S-[2-[3-[[(2R)-4-[[[(2R,3S,4R,5R)-5-(6-aminopurin-9-yl)-4-oxidanyl-3-phosphonooxy-oxolan-2-yl]methoxy-oxidanyl-phosphoryl]oxy-oxidanyl-phosphoryl]oxy-3,3-dimethyl-2-oxidanyl-butanoyl]amino]propanoylamino]ethyl] 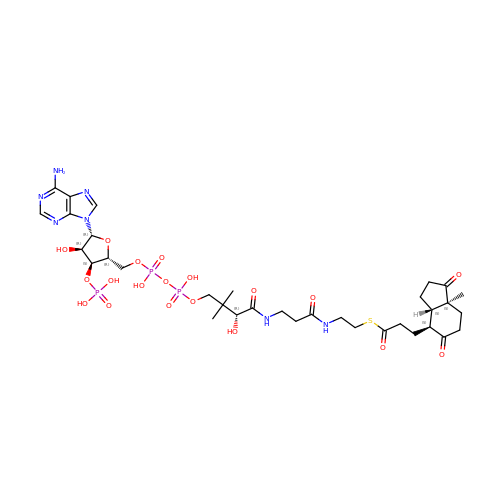3-[(3aS,4S,7aS)-7a-methyl-1,5-bis(oxidanylidene)-2,3,3a,4,6,7-hexahydroinden-4-yl]propanethioate | C34 H52 N7 O19 P3 S | IWNWMTZIJPUDPV-MDQHZGBLSA-N> MKVAVLPGDGIGPEVTEAALKVLRALDEAE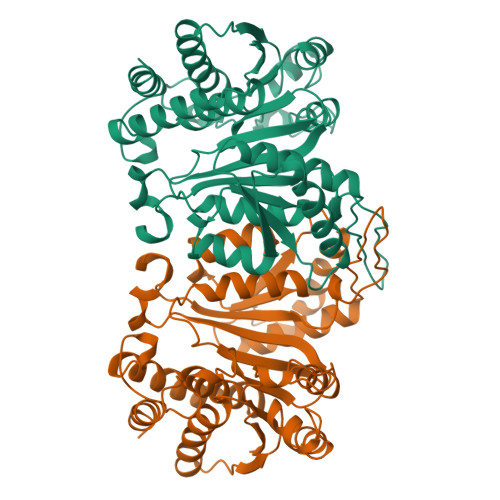GLGLAYEVFPFGGAAIDAFGEPFPEPTRKGVEEAEAVLLGSVGGPKWDQNPRELRPEKGLLSIRKQLDLFANLRPVKVFESLSDASPLKKEYIDNVDFVIVRELTGGIYFGEPRGMSEAEAWNTERYSKPEVERVARVAFEAARKRRKHVVSVDKANVLEVGEFWRKTVEEVGRGYPDVALEHQYVDAMAMHLVRSPARFDVVVTGNIFGDILSDLASVLPGSLGLLPSASLGRGTPVFEPVHGSAPDIAGKGIANPTAAILSAAMMLEHAFGLVELARKVEDAVAKALLETPPPDLGGSAGTEAFTATVLRHLA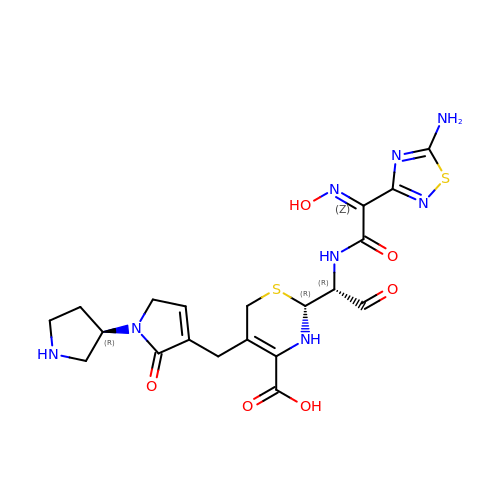(2R)-2-[(1R)-1-{[(2Z)-2-(5-amino-1,2,4-thiadiazol-3-yl)-2-(hydroxyimino)acetyl]amino}-2-oxoethyl]-5-({2-oxo-1-[(3R)-pyrrolidin-3-yl]-2,5-dihydro-1H-pyrrol-3-yl}methyl)-3,6-dihydro-2H-1,3-thiazine-4-carboxylic acid | C20 H24 N8 O6 S2 | MYAXGJQBOYOEHQ-SWBIIUODSA-N>GHMEQTHRAIFRFVPRHEDELELEVDDPLLLELQAEDYWYEAYNMRTGARGVFPAYYAIEVTK[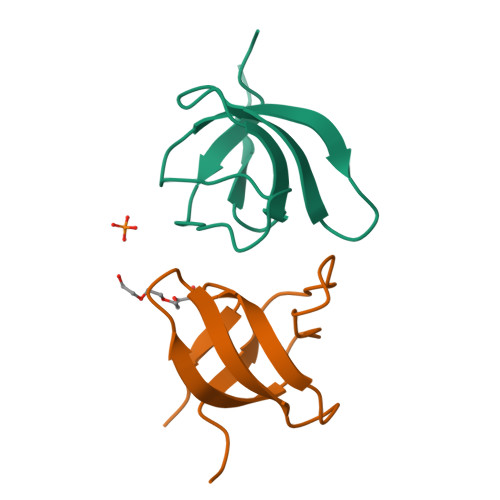12x]>LGFSFEFTEQQKEFQATARKFAREEIIPVAAEYDKTGEYPVPLIRRAWELGLMNTHIPENCGGLGLGTFDACLISEELAYGCTGVQTAIEGNSLGQMPIIIAGNDQQKKKYLGRMTEEPLMCAYCVTEPGAGSDVAGIKTKAEKKGDEYIINGQKMWITNGGKANWYFLLARSDPDPKAPANKAFTGFIVEADTPGIQIGRKELNMGQRCSDTRGIVFEDVKVPKENVLIGDGAGFKVAMGAFDKTRPVVAAGAVGLAQRALDEATKYALERKTFGKLLVEHQAISFMLAEMAMEVELARMSYQRAAWEVDSGRRNTYYASIAKAFAGDIANQLATD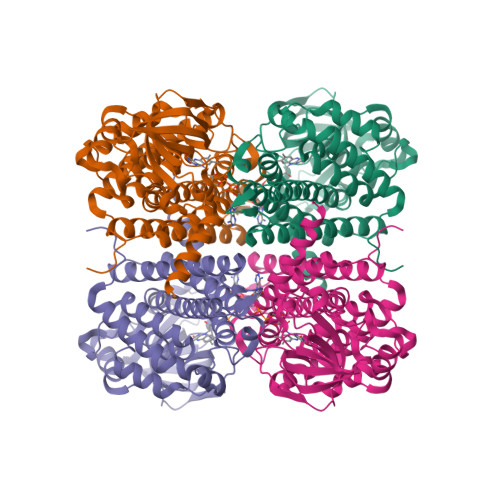AVQILGGNGFNTEYPVEKLMRDAKIYQIYEGTSQIQRLIVAREHIDKYKN[4x]The Minichromosome Maintenance (MCM) complex forms an essential hexameric-ring helicase that unwinds DNA at the replication fork (1–3). MCM proteins have three conserved domains: an N-terminal domain (MCMN) that mediates the head-to-head interaction of the initial double-hexamer; a conserved AAA+ ATPase domain; and a short helix-turn-helix domain at the C-terminus. Crystal structures of the N-terminal domains of Methanobacterium thermautotrophicus (MtMCMN), Sulfolobus solfataricus (SsoMCMN) and Pyrococcus furiosis (PfMCMN) show a consistent hexameric ring structure with three subdomains: a helical subdomain-A, a Zn-binding subdomain-B and an OB-fold subdomain-C. The crystal structure of PfMCMN bound to single-stranded DNA (ssDNA) revealed that subdomain-C binds ssDNA in the plane of the hexameric ring via conserved residues defined as the MCM single-stranded DNA-binding motif (MSSB).

One mutant is a triple-mutant of the PfMCMN β-turn, K233A/R234A/K236A (PfMCMN-βT). The crystal structure of PfMCMN-βT consists of a central pentameric ring with five peripheral monomers. As in the PfMCMN-WT hexamer, adjacent subunits interact with each other via a short antiparallel β-sheet interaction: P130 carbonyl–F240 amide and V132 amide–P238 carbonyl. Intriguingly, two of the residues involved in this interaction, P238 and F240, are positioned just following the 3 alanine mutations on the β-turn, providing a straightforward basis for the different oligomeric form of PfMCMN-βT than the PfMCMN-WT hexamer. In particular, the carbonyl of P238 is notably shifted in PfMCMN-βT when compared to PfMCMN-WT. This shift is not compatible with retaining the specific P238-V132 interaction in a hexamer because the constituent atoms are separated by 4 Å when PfMCMN-βT monomers are superimposed on each subunit of the wild-type hexamer (data not shown). AUC sedimentation velocity and equilibrium experiments show that PfMCMN-βT most likely adopts a pentameric structure in solution. Analysis with an A5 ↔ 5A model (where A5 is pentamer and A is monomer) indicates that the protein concentration where 50% is pentameric and 50% is monomeric (Kd1–5 = 8 μM) is 7-fold lower than that of the PfMCMN-WT hexamer (Kd1–6 = 60 μM). The PfMCMN-βT mutant forms a pentameric ring that does not bind ssDNA. A pentamer, therefore, may not be able to attain the precise interface needed to bind ssDNA.

>SVDREEMIERFANFLREYTDEDGNPVYRGKITDLLTITPKRSVAIDWMHLNSFDSELAHEVIENPEEGISAAEDAIQIVLREDFQREDVGKIHARFYNLPETLMVKDIGAEHINKLIQVEGIVTRVGEIKPFVSVAVFVCKDCGHEMIVPQKPYESLEKVKKCEQCGSKNIELDVNKSSFVNFQSFRIQDRPETLKGGEMPRFIDGILLDDIVDVALPGDRVIVTGILRVVLEAAEATPIFRKILEVNHIEPVSKEI[10x]>[2x]TRDANGTWEMESNENFEGWMKALDIDFALRKIAVRLTQTLVIDQ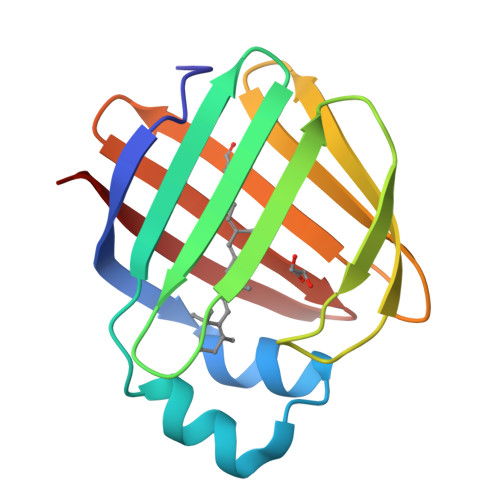DGDNFKVKCTSTFWNYDVDFTVGVEFDEYTKSLDNRHVKALVTWEGDVLVCVQKGEKENRGWKKWIEGDKLYLELTCGDQVCRQVFKKK> HPETLVKVKDAEDQLGGRVGYIELDLASGKILESFRPEERFPMMSTFKVLLCGAVLSRVDAGQEQLGRRIHYSQNDLVEYSPVTEKHLTDGMTVGELCSAAITMSDNTAANLLLTTIGGPKELTAFLHNMGDHVTRLDSWEPELNEAIPNDERDTTTPVAMATTLRKLLTGELLTAASRQQLIDWMEADKVAGPLLRSALPAGWFIADKSGASERGSRGIIAALGPDGKPSRIVVIYMTGSQATMDERNRQIA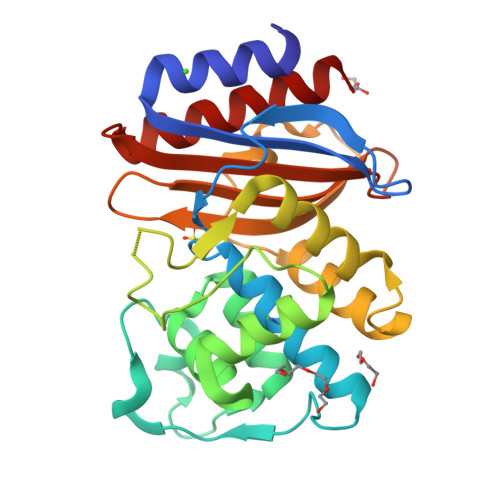EIGASLIKHW>[2x]GMAN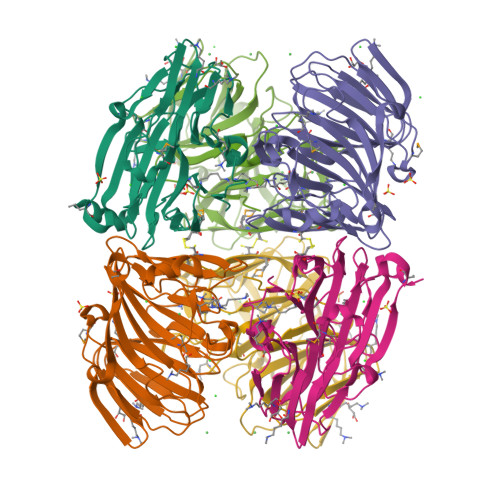LLSTCTSESGNIQHISPQNAGWEYVGFDVWQLKAGESITLPSDERERCLVLVAGLASVKAADSFFYRIGQRMSPFERIPAYSVYLPHHTEAKVTAETDLELAVCSAPGFGELPVRLISPQEVGVEHRGKGRNQRLVHNILPDSQLADSLLVVEVYTNAGATSSWPAHKHDTAVEGQETYLEETYYHRFNPPQGFCLQRVYTDDRSLDECMAVYNRDVVKVPKGYHPVATIAGYDNYYLNVMAGPLRKWRFTWEENHAWINSPDYPR> ASSVNELENWSKWMQPIPDSIPLARISIPGTHDSGTFKLQNPIKQVWGMTQEYDFRYQMDHGARIFDIRGRLTDDNTIVLHHGPLYLYVTLHEFINEAKQFLKDNPSETIIMSLKKEYEDMKGAEDSFSSTFEKKYFVDPIFLKTEGNIKLGDARGKIVLLKRYSGSNEPGGYNNFYWPDNETFTTTVNQNANVTVQDKYKVSYDEKVKSIKDTMDETMNNSEDLNHL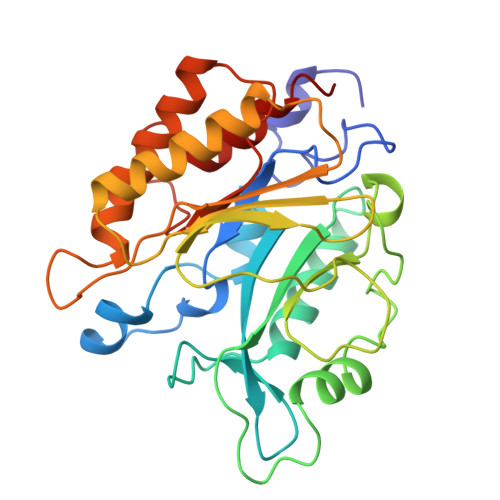YINFTSLSSGGTAWNSPYYYASYINPEIANYIKQKNPARVGWVIQSYINEKWSPLLYQEVIRANKSLIKE> PPAQLSVHTVSWNSGHERVPTNLEELLGLNSGETPDVIAVAVQGFGFQTDKPQQGPACVKNFQSLLTSKGYTKLKNTITETMGLTVYCLEKHLDQNTLKNETIIVTVDDQKKSGGIVTSFTIYNKRFSFTTSRMSDEDVTSTNTKYAYDTRLDYSKKDDPSDFLFWIGDLNVRVETNATHAKSLVDQNNIDGLMAFDQLKKAKEQKLFDGWTEPQVTFKPTYKFKPNTDEYDLSATPSWTDRALYKSGTGKTIQPLSY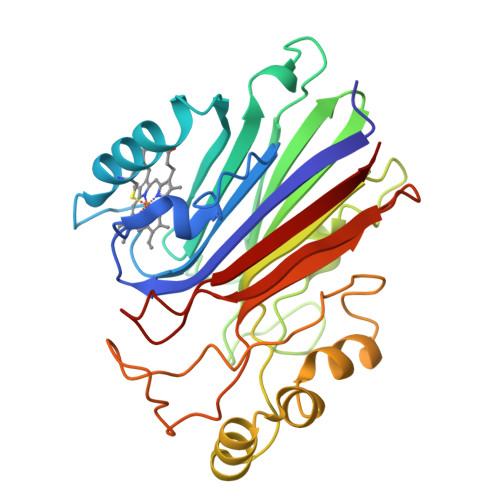NSLTNYKQTEHRPVLAKFRVTL> MGSSHHHHHHMPFTIDSARGIFPNTLAADVVPATIARFSQLNAEDQLALIWFAYLEMGKTLTIAAPGAASMQLAENALKEIQAMGPLQQTQAMCDLANRADTPLCRTYASWSPNIKLGFWYRLGELMEQGFVAPIPAGYQLSANANAVLATIQGLESGQQITVLRNAVVDMGFTAGKDGKRIAEPVVPPQDTASRTKVSIEGVTNATV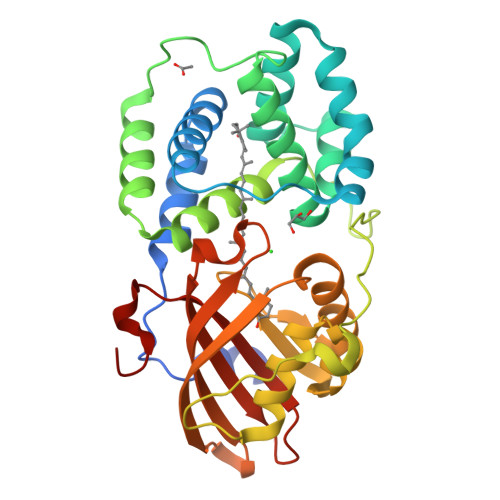LNYMDNLNANDFDTLIELFTSDGALQPPFQRPIVGKENVLRFFREECQNLKLIPERGVTEPAEDGFTQIKVTGKVQTPWFGGNVGMNIAWRFLLNPEGKIFFVAIDLLASPKELLNFAR>GAMVTRLRQRIDAAVAQFADSGLRTSVQFVGPLSVVDSALADQAEAVVREAVSNAVRHAAASTLTVRVKVDDDLCIEVTDNGRGMPDEFTGSGLTNLRQRAEQAGGEFTLAS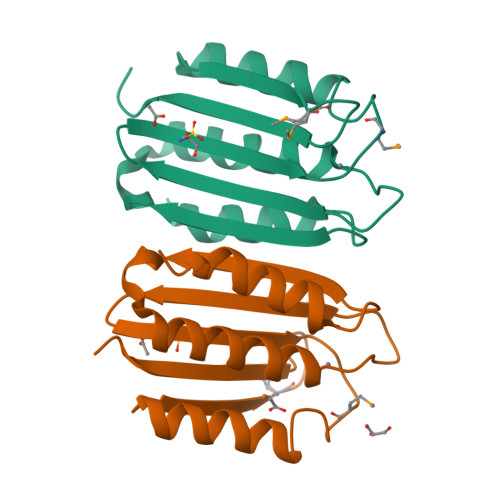MPGASGTVLRWSAPLSQ[2x]>[3x]STNDNIKDLL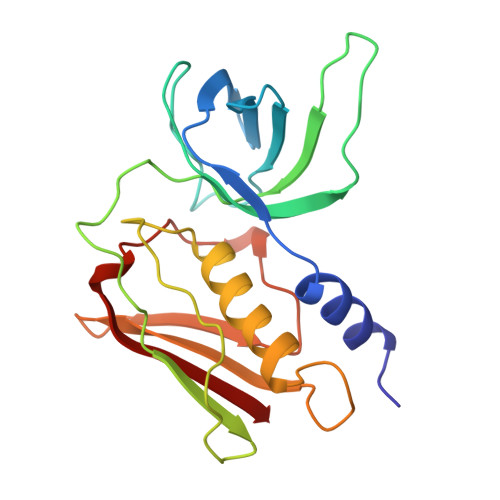DWYSSGSDTFTNSEVLDNSLGSMRIKNTDGSISLIIFPSPYYSPAFTKGEKVDLNTKRTKKSQHTSEGTYIHFQISGVTNTEKLPTPIELPLKVKVHGKDSPLKYWPKFDKKQLAISALDFEIRHQLTQIHGLYRSSDKTGGYWKITMNDGSTYQSDLSKKFEYNTEKPPINIDEIKTIEAEIN(3~{R})-3-[3-[2-aminocarbonyl-6-(trifluoromethyloxy)indol-1-yl]phenyl]butanoic acid | C20 H17 F3 N2 O4 | 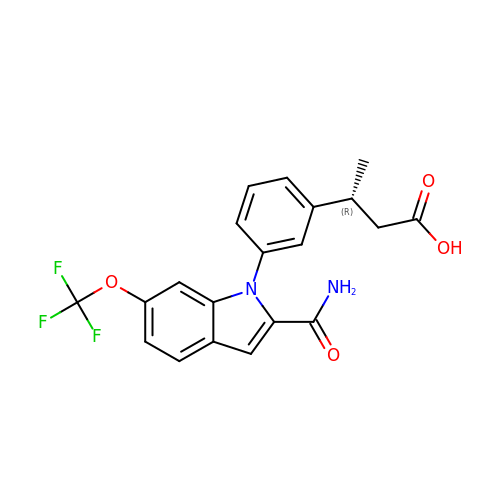OSJXLDOVNXZNHD-LLVKDONJSA-N>[2x]MGSLDTNPTAFSAFPAGEGETFQPLNADDVRSYLHKAVDFISDYYKSVESMPVLPNVKPGYLQDELR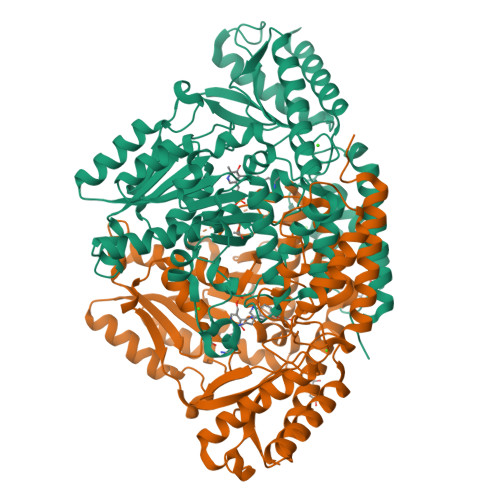ASPPTYSAPFDVTMKELRSSVVPGMTHWASPNFFAFFPSTNSAAAIAGDLIASAMNTVGFTWQASPAATEMEVLALDWLAQMLNLPTSFMNRTGEGRGTGGGVILGTTSEAMLVTLVAARDAALRRSGSDGVAGLHRLAVYAADQTHSTFFKACRLAGFDPANIRSIPTGAETDYGLDPARLLEAMQADADAGLVPTYVCATVGTTSSNAVDPVGAVADVAARFAAWVHVDAAYAGSACICPEFRHHLDGVERVDSISMSPHKWLMTCLDCTCLYVRDTHRLTGSLETNPEYLKNHASDSGEVTDLKDMQVGVGRRFRGLKLWMVMRTYGVAKLQEHIRSDVAMAKVFEDLVRGDDRFEVVVPRNFALVCFRIRAGAGAAAATEEDADEANRELMERLNKTGKAYVAHTVVGGRFVLRFAVGSSLQEEHHVRSAWELIKKTTTEMMN>[2x]MVARVQTAEEIRDEGNAAVKDQDYIKADELYTEALQLTTDEDKALRPVLYRNRAMARLKRDDFEGAQSDCTKALEFDGADVKALFRRSLAREQLGNVGPAFQDAKEALRLSPNDKGIVEVLQRLVKANNDKIKQTTSLANKVTDMEKLAFRGEAKDTEQKMTALNNLLVLCRESESGATGVWNQGALVPFVLNLINDASENEEVTVTAIRILDETIKNSVRCMKFLAMHDPDGPKSVRFVCRLMCKKSTKDFVDATG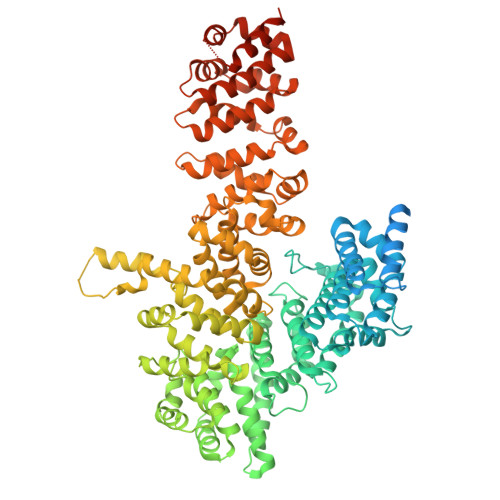ILVQRVFNAMAKMDRQKEMKPDPEVAEANKIWIIRVLLELQEMLQDPKVGAVQRETCIDLFLKNLMHMDGGIPRGWSWKFVEERGLLALLDVASQIPELCEYPVSAETRQHVAICLQRLEEDMVFDTKRTIFKEKVDMFFNALISRCTNDDEGHKYRIKLSCFLITMLQGPVDIGINLITNDQLTPIMLEMAASQDHLMQGIAAELIVATVSKHERAINMLKVGIPVLRALYDSEDPTVKVRALVGLCKIGAAGGDDISKATMKEEAVISLAKTCKKFLLETEKYSVDIRRYACEGLSYLSLDADVKEWIVDDSLLLKALVLLAKKAGALCVYTLATIYANLSNAFEKPKVDEEMVKLAQFAKHHVPETHPKDTEEYVEKRVRALVEEGAVPACVAVSKTESKNALELIARSLLAFAEYEDLRGRIIAEGGTVLCLRLTKEASGEGKIKAGHAIAKLGAKADPMISFPGQRAYEVVKPLCDLLHPDVEGKANYDSLLTLTNLASVSDSIRGRILKEKAIPKIEEFWFMTDHEHLRAAAAELLLNLLFFEKFYEETVAPGTDRLKLWVLYSAEVEEERLSRASAAGFAILTEDENACARIMDEIKSWPEVFKDIAMHEDAETQRRGLMGIANIMHSSNKLCSEIVSSEVFRVLVAVTKLXXXXXXXXXXXXXXXXXXXXXXXXXXXXXXXXXXXXXXXXXXXXXXXX>MTMRSTNWAGNVVYRASELHRPASLDELRRVVARSPKVRVLGSGHSFNEITDTEGALVSLEALPPEVEIDRATGTARVAAGLRYGELSARLHAAGYALPNLASLPHICVAGACATGTHGSGDGIGGLAGSVTAVELVTADGDLVTLSRDADPDRFPGAVVSLGALGAVVTMTLRLEPAFQVRQRVYENLPAEALDDHFDEIMASGYSVSLFTDWRGDRIRQVWVKERVGDPAAGGEEREPVVAALGATPADGPRHPVPGMPAANCTEQLGVPGPWHERLPHFRLGFTPSSGDELQAEYLLPRRHAVAAFHALAGIADRIAPVLHISEIRTVAADDLWLSPFHGRNTVAFHFTWKPDEAAVREVLSLMEEVLAPFEPRPHWGKLFAIPPKVLRSRYDRIGDFRALARELDPSGKFANAFVAHHVLDDE[4x]

Alditol oxidases are promising tools for the biocatalytic oxidation of glycerol to more valuable chemicals. On the other hand, certain alditol oxidases (AldO; EC 1.1.3.41) were found to be moderately active on glycerol without being affected by the inactivating semiquinone formation. Three thermostable alditol oxidases from Actinobacteria Bacterium, Streptomyces thermoviolaceus, and Thermostaphylospora chromogena active on glycerol were discovered. The characterization of these three flavoenzymes demonstrated their glycerol oxidation activities, preference for alkaline conditions, and excellent thermostabilities with melting temperatures higher than 75 °C. Structural elucidation of the alditol oxidase from Actinobacteria Bacterium highlighted a constellation of side chains that engage the substrate through several hydrogen bonds, a histidine residue covalently bound to the FAD prosthetic group, and a tunnel leading to the active site.

AldOAb was crystallized with xylulose, the product of xylitol oxidation. The overall structural assembly is composed by 14 α helices and 14 β sheets that are organized into two distinct domains, as observed in other members of the VAO family: an FAD-binding domain and a substrate-binding domain. The planar flavin cofactor sits at the domain interface with its 8α-methyl group covalently bound to the Nδ1 of His45. The residues that compose the active site wrap the isoalloxazine on its re side. They include Gln295, Glu327, Arg329, His350, and Lys382 belonging to the substrate binding domain, and Ser103, His118, and His45 being part of the FAD binding domain. A well-ordered molecule of D-xylulose, present in the reservoir solution of the crystallization condition, was clearly visible in the electron density. The ligand is buried in the catalytic pocket, and its OH groups are engaged in H-bonds with the surrounding side chains. His350 and Lys382 are located at the bottom of the substrate site where they interact with the C1-O1 group of the D-xylulose bound in front of the reactive N5 atom of the flavin. This geometry is perfectly suited for the hydride transfer from the substrate C1 carbon leading to aldehyde or carboxylic (e.g., glycerate from glycerol) products as observed in the AldO enzymes so-far characterized. When inspecting the molecular surface of AldOAb, a noticeable feature is the presence of a wide tunnel that connects the active site to the external surface. With a diameter of about 10 Å and a length of 14 Å, the tunnel is long and wide enough to bind polyols of different lengths and sizes.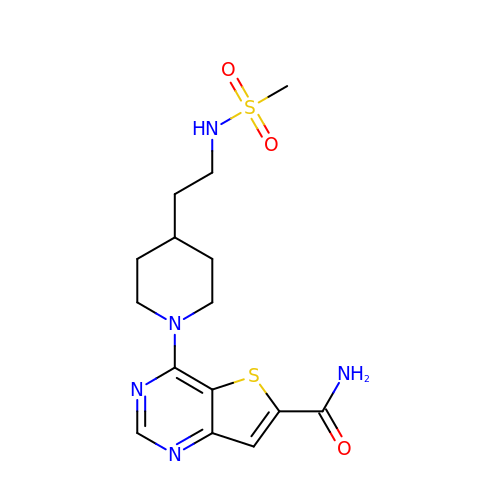4-(4-{2-[(methylsulfonyl)amino]ethyl}piperidin-1-yl)thieno[3,2-d]pyrimidine-6-carboxamide | C15 H21 N5 O3 S2 | BKOWIHMCGFRARN-UHFFFAOYSA-N>MSSGGDPSEDTGAGDGEQGGESSAMAGRSGGGMGGGGGGGGSVGFSTGGWEGGTYFSDHTVTTTNTRQWYTGILNGHRYSKLAQTTGSNLQAAKPWVGIQTPWAYLNLNCYHCHFSPQDWQRLLNEYKAWRPKRMHVRIYNLQIKQITTVGADTLYQNDLTAGVHIFCDGSHQYPYAQHPWDEGASPELPNEIWKLPQYAYFQYQGDLTDHATANTPQNVESMLRSNIPLFLLENSNHEVLRTGEMTEFSFTFQSGWVTNDRAYCCPQSDFNPLVQTRRYYPTWNGSSNSYSYNRYGPYKKPSNWMPGPGLAYKGATHTNQNPDDARGPIVTTIAPRGTISVGSTPSNDAPNDGDNTISSDGVKQGGWQTAPVNGACSRTDYPTLAFDPSDRSTNQNIPTRNLDIDMTRWYRVHEPVRSGNGSTYYNVDDVWMYPNQVWNSTPICRDNPIWDKVPRTDHHTLLDSSDGTLPMKHPPGNIFIKCAKIPIPTSNNTDSYLNIYVTGQVTYTVEWEVQRYQTKNWRPELRTSAGTYNQHEIYNIGENGTYNRANTFNECMPTKCGINRVL[60x]

To expand the structural repertoire of determined capsid structures for the diverse Bocaparvovirus genus, viruses infecting dogs (CnMV), pigs (PBoV1), and rats (RBoV) were selected. The ORFs of these viruses coding for the major capsid protein VP2 were cloned into the pFastBac1 plasmid to enable the production of the virus-like particles (VLPs), using the Bac-to-Bac expression system in insect Sf9 cells. In the icosahedral capsid, the 60 VPs assemble via two-, three-, and fivefold symmetry-related VP interactions, resulting in pores at the fivefold symmetry axes, protrusions surrounding the threefold axes, and depressions at the twofold axes.

The first porcine bocavirus (PBoV) was identified in Swedish pigs in 2009. PBoV is usually associated with diarrhea and upper respiratory tract infections in piglets, but a case study in 2016 associated PBoV with a case of encephalomyelitis in a 6-week-old piglet in Germany. The capsid (VP1) amino acid sequence identity of PBoV1 is 42% and 47% for BPV and HBoV1, respectively. Following cryo-EM data collection, three-dimensional-image reconstruction of the capsids, utilizing 50,866 (CnMV), 98,388 (PBoV1), and 9199 (RBoV) individual capsid images, resulted in a resolution of 2.72, 2.31, and 2.52 Å, respectively. The high resolution of the cryo-EM maps allowed the building of reliable atomic models, starting from amino acids 34, 41, and 42 (VP2 numbering) at the N-terminus for CnMV, PBoV1, and RBoV, respectively. In the case of PBoV1 and RBoV, the cryo-EM maps for the most part also showed densities for the carbonyl groups of the main-chain and densities for a specific rotamer for the individual amino acids, guiding the model building for these viruses. Capsid structures previously determined for the Bocaparvovirus genus showed disperse protrusions surrounding the threefold axis that do not significantly extend radially from the capsid surface. In contrast, the CnMV capsid shows very prominent threefold protrusions, while PBoV1 and RBoV follow the previously described characteristics of the genus. In PBoV1 and RBoV, the shorter VR-III does not cover the entire twofold region, but their loop also advances the twofold axis and restricts the size of the depression. Another feature previously observed for the bocaviruses, with the exception of GBoV1, was the presence of density extending into the interior of the capsid below the fivefold channel. This density was also seen for CnMV, but is absent in the PBoV1 and RBoV capsids.> GAMTFTRYSRLRVIAEIRHGDIFHSANIVSSIEFDRDDELFATAGVSRCIKVFDFSSVVNEPADMQCPIVEMSTRSKLSCLSWNKHEKNHIASSDYEGIVTVWDVTTRQSLMEYEEHEKRAWSVDFSRTEPSMLVSGSDDCKVKVWCTRQEASVINIDMKANICCVKYNPGSSNYIAVGSADHHIHYYDLRNISQPLHVFSGHKKAVSYVKFLSNNELASASTDSTLRLWDVKDNLPVRTFRGHTNEKNFVGLTVNSEYLACGSETNEVYVYHKEITRPVTSHRFGSPDMDDAEEEAGSYFISAVCWKS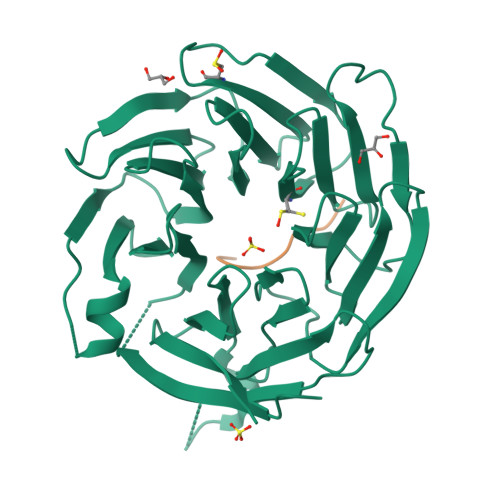DSPTMLTANSQGTIKVLVLAA;> XGFGVVPSFY>MAKVTELGYLGLSVSNLDAWRDYAAGIMGMQVVDDGEDDRIYLRMDRWHHRIVLHADGSDDLAYIGWRVAGPVELDELAEQLKNAGIPFEVASDADAAERRVLGLVKLHDPGGNPTEIFYGPQVDTSSPFHPGRPMFGKFVTEGQGLGHIIIREDDVEEATRFYRLLGLEGAVEYKFALPNGAVGTPVFMHCNDRHHSLAFGVGPMDKRINHLMIEYTHLDDLGYAHDLVRQQKIDVTLQIGKHSNDEALTFYCANPSGWLWEPGWGSRPAPAQQEHYLRDIFGHDNEVEGYGLDIPLKGLDIPA[4x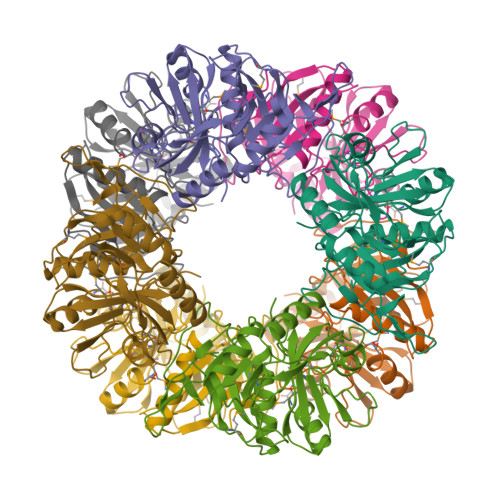]>[2x]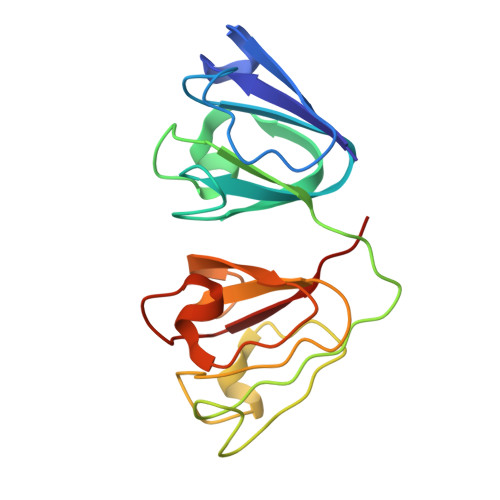GKITLYEDRGFQGRHYECSSDHPNLQPYLSRCNSASVDSGCWMLYEQPNYSGLQYFLRRGDYADHQQWMGLSDSVRSCRLIPHSGSHRIRLYEREDYRGQMIEFTEDCSCLQDRFRFNEIHSLNVLEGSWVLYELSNYRGRQYLLMPGDYRRYQDWGATNARVGSLRRVIDFS>MENFPTEYFLNTTVRLLEYIRYRDSNYTREERIENLHYAYNKAAHHFAQPRQQQLLKVDPKRLQASLQTIVGMVVYSWAKVSKECMADLSIHYTYTLVLDDSKDDPYPTMVNYFDDLQAGREQAHPWWALVNEHFPNVLRHFGPFCSLNLIRSTLDFFEGCWIEQYNFGGFPGSHDYPQFLRRMNGLGHCVGASLWPKEQFNERSLFLEITSAIAQMENWMVWVDDLMSFYKEFDDERD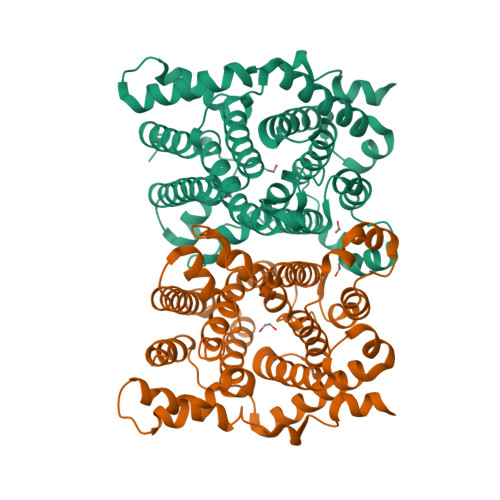QISLVKNYVVSDEISLHEALEKLTQDTLHSSKQMVAVFSDKDPQVMDTIECFMHGYVTWHLCDRRYRLSEIYEKVKEEKTEDAQKFCKFYEQAANVGAVSPSEWAYPPVAQLANVRSKDVKEVQKPFLSSIELVE[2x]> ACDYTCGSNCYSSSDVSTAQA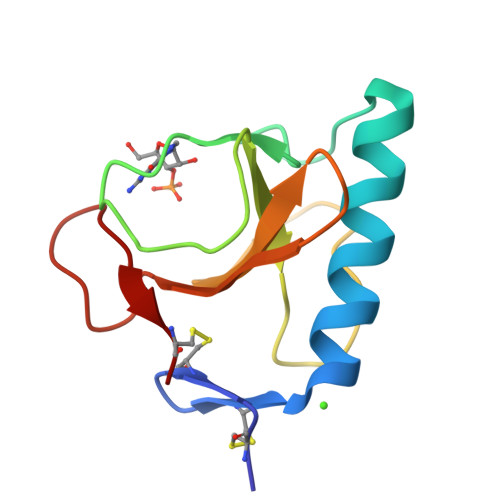AGYKLHEDGETVGSNSYPAKYNNYEGFDFSVSSPYYAWPILSSGDVYSGGSPGADRVVFNENNQLAGVITHTGASGNNFVECT>GHMEQTHRAIFRFVPRHEDELELEVDDPLLAELQAEDYWYEAYNMRTGARGVFPAYYAIEVTK[4x]

Aromatic residues cluster in the core of folded proteins, where they stabilize the structure through multiple interactions. NMR studies in the 1970s demonstrated that aromatic side chains can undergo ring flips—that is, 180° rotations of the χ2 dihedral angle (Cβ–Cγ axis)—even when engaged in stabilizing interactions in the hydrophobic core. Here we capture ring flipping events of a buried tyrosine residue in the SH3 domain of the JNK-interacting protein 1 (JIP1). Our data therefore suggest that the conformation of the aromatic ring at position 526 is determined by steric interactions dictated by the size of the surrounding amino acids.

Accordingly, we designed four different mutants of JIP1-SH3 (H493A, V517A, V517L and A541L) and obtained their high-resolution structures by X-ray crystallography. Of note, three mutants (H493A, V517A and A541L) induce a staggered conformation of Y526, with χ2 dihedral angles ranging from −41° to −75°, whereas V517L shows an eclipsed conformation of Y526 and an almost identical structure to the wild-type protein. The H493A and V517A variants show almost identical crystal structures and for a subset of residues, the chemical shifts of which are unaffected by the mutations, the resonances of the two variants fall on a straight line together with the resonances of the wild-type protein. This suggests that they are in fast–intermediate exchange between two conformations represented by the crystal structures of the wild-type protein and of the H493A/V517A variants. In agreement with this, both variants show line broadening and chemical exchange contributions as detected by 15N and 1HN relaxation dispersion. Analysis of these data shows that the structural features of the minor state of the wild-type protein are captured by the H493A/V517A crystal structures, as shown by the excellent agreement between the ΔδCPMG values for the wild-type protein and the two variants. In addition, the analysis yields exchange rates between the staggered (canonical β-strand) and the eclipsed (classic β-bulge) conformation of kEX = 2,830 ± 70 s−1 (H493A) and kEX = 6,800 ± 300 s−1 (V517A), compared to kEX = 2,600 ± 70 s−1 determined for the wild-type protein. Finally, the observable chemical shifts of the two variants, in conjunction with analysis of the relaxation dispersion data (Supplementary Discussion), show that the H493A mutation slightly stabilizes the minor state relatively to the major state, whereas the V517A mutation almost inverts the relative populations of the major and minor states.> PVTDAYWQILFSVLKVTRNLKELDLSGNSLSHSAVKSLCKTLRRPRCLLETLRLAGCGLTAEDCKDLAFGLRANQTLTELDLSFNVLTDAGAKHLCQRLRQPSCKLQRLQL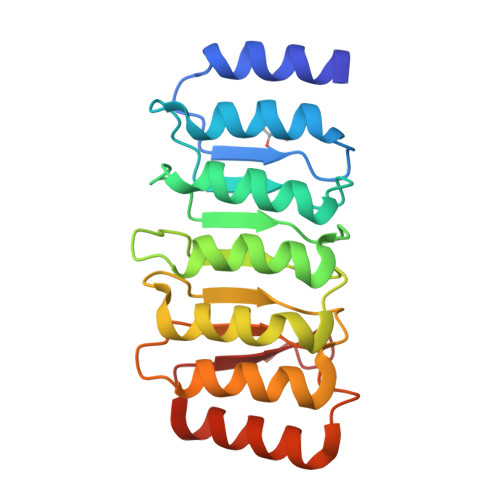VSCGLTSDCCQDLASVLSASPSLKELDLQQNNLDDVGVRLLCEGLRHPACKLIRLGLDQTTLSDEMRQELRALEQEKPQLLIFSRRKPS>SEGSDAPNFVLEDTNGKRIELSDLKGKGVFLNFWGTWCEPCKKEFPYMANQYKHFKSQGVEIVAVNVGESKIAVHNFMKSYGVNFPVVLDTDRQVLDAYDVSPLPTTFLINPEGKVVKVVTGTMTESMIHDYMNLIKPGETSGL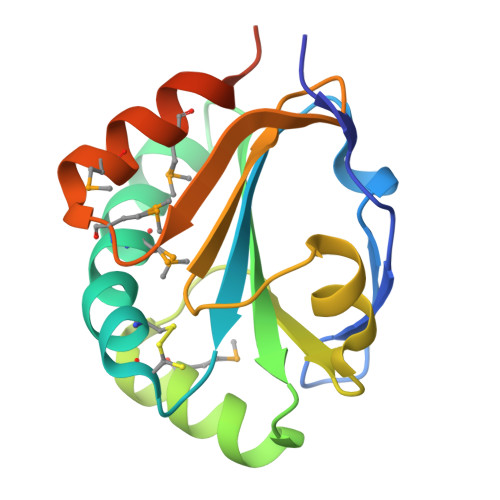EHHHHHH[2x]>[5x]MNLTELKNTPVSELITLGENMGLENLARMRKQDIIFAILKQHAKSGEDIFGDGVLEILQDGFGFLRSADSSYLAGPDDIYVSPSQIRRFNLRTGDTISGKIRPPKEGERYFALLKVNEVNFDKPENARNKILFENLTPLHANSRLRMERGNGSTEDLTARVLDLASPIGRGQRGLIVAPPKAGKTMLLQNIAQSIAYNHPDCVLMVLLIDERPEEVTEMQRLVKGEVVASTFDEPASRHVQVAEMVIEKAKRLVEHKKDVIILLDSITRLARAYNTVVPASGKVLTGGVDANALHRPKRFFGAARNVEEGGSLTIIATALIDTGSKMDEVIYEEFKGTGNMELHLSRKIAEKRVFPAIDYNRSGTRKEELLTTQEELQKMWILRKIIHPMGEIDAMEFLINKLAMTKTNDDFFEMMKRS;>[4x]AMGNDTYQPINCDDYDNLELACQHHLMLTLELKDGEKLQAKASDLVSRKNVEYLVVEAAGETRELRLDKITSFSHPEIGTVVVSES

Bacterial transcription termination factor, ρ, is a hexameric, NTP-dependent 5’–3’ RNA translocase and helicase. A ρ monomer contains N-terminal (NTD) and C-terminal (CTD) domains connected by a flexible linker. The NTD comprises an N-terminal three-helix bundle and a five-stranded β-barrel, the OB-fold, that forms a primary RNA-binding site (PBS); the PBSes are located around one outer rim of the ρ hexamer. The CTDs jointly form a secondary RNA-binding site (SBS) at the center of the ρ hexamer.

We subjected SEC fractions corresponding to ρ-Rof complexes to cryoEM/SPA in the absence and presence of the transition state analog, ADP-BeF3. Multi-particle 3D refinement with ~600,000 particle images yielded two cryoEM reconstructions for each sample, corresponding to two ρ-Rof assemblies. In the first assembly, ρ forms an open hexameric ring (ρA-ρF) bound by five Rof molecules (Rofa-Rofe), while the second assembly represents a ρ pentamer (ρA-ρE) bound by four Rof molecules (Rofa-Rofd). In the presence of ADP-BeF3, we obtained a ~1:1 (ρ6-Rof5:ρ5-Rof4) distribution between the two classes, whereas in the absence of the nucleotide, the equilibrium was shifted towards the lower oligomeric assembly (ρ6-Rof5:ρ5-Rof4 ~ 1:3). The reconstructions do not reveal differences in the ρ-Rof interfaces, irrespective of oligomeric state or bound nucleotide. The local resolutions of the reconstructions decrease towards the regions corresponding to terminal ρ subunits and bound Rof. Weaker density for the peripheral Rof molecules could indicate a higher flexibility or a lower occupancy. Rof molecules are bound between protomers ρA-ρB, ρB-ρC, etc., but not preceding or following the terminal ρ subunits, ρA and ρF.>MSAKSRTIGIIGAPFSKGQPRGGVEEGPTVLRKAGLLEKLKEQECDVKDYGDLPFADIPNDSPFQIVKNPRSVGKASEQLAGKVAEVKKNG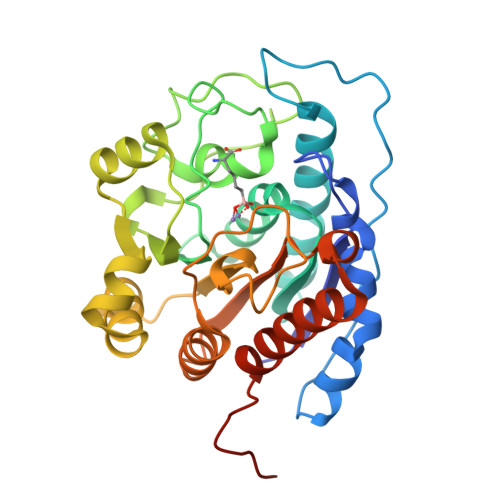RISLVLGGDHSLAIGSISGHARVHPDLGVIWVDAHTDINTPLTTTSGNLHGQPVSFLLKELKGKIPDVPGFSWVTPCISAKDIVYIGLRDVAPGEHYILKTLGIKYFSMTEVDRLGIGKVMEETLSYLLGRKKRPIHLSFDVDGLDPSFTPATGTPVVGGLTYREGLYITEEIYKTGLLSGLDIMEVNPSLGKTPEEVTRTVNTAVAITLACFGLAREGNHKPIDYLNPPK[2x]> GPKGTEKTVKVIKDGPALGLTISDNG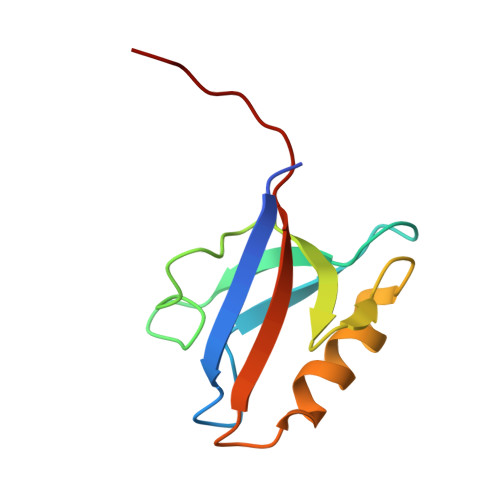AGYAFIKKIREDSIMSRVANVAVGDHIAKINGTDLNGCRHFEVARMLKEIPIGSEFTMICVEPKKSESKV>[7x]MIMDKENTFSYKQAITGTAVSTNVIDLGVSRDIGKGVPVPIIIQVVEDFADATSLTATLQTSETENFSSATTLATSGAVPVADLTAGKQLAVQYMPLGTQRYLRVNYTVSGTATAGAVTAGVVMSHQQND;>MATLGNTYLTLADVQKQKDGKGNVTSEIIEMLAETNPILEDMVVMECNDGTGHLTTIRTGL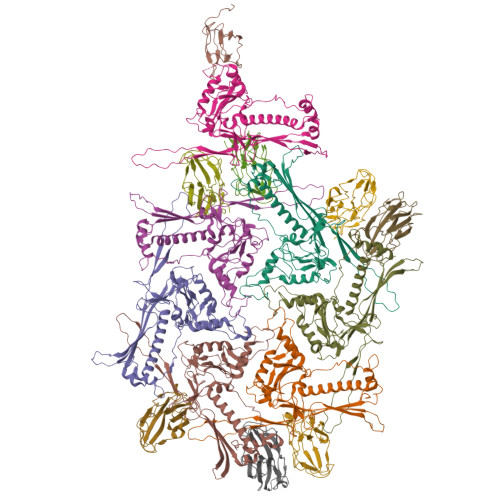PQATWRRLYEGVQPAKSTTRQIKDSTGTLEAWSEVDEKLVKLSKDKQQLMLNEAAAFLEGMNQTMASTLFYGNTATDAVKFMGLAPRFNAYRAARNLKPVDTADQVIDAGGTGSDLTSIWMVVWGDRTAHGLYPEGTSAGLQREYLGAETKELGDGGVYRVVREKFEWDLGLTVRDFRYVVRIANIDVSDLQAGTIDIYALLRKAYYRLENRVITGGRAALYCNADVTEAMDAAATPTSSTTASYVRLTPMQVDGKEVMMYRGIPVRECDAILSTETAVPSVA[7x];> MAIGDIQTSVAFDRQVGRFPPRAEVVTPSNSEEFTSGVSVFSNDGGDISVVPLLPYGSAAIVVTVAAGGFVPFMVRKVNATGTTSTSIVAVW>GSHMAGIFDLSGRKAIVTGGSKGIGAAIARALDKAGAT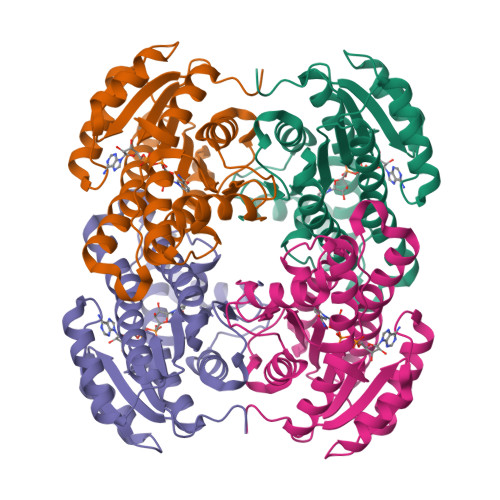VAIADLDVMAAQAVVAGLENGGFAVEVDVTKRASVDAAMQKAIDALGGFDLLCANAGVSTMRPAVDITDEEWDFNFDVNARGVFLANQIACRHFLASNTKGVIVNTASLAAKVGAPLLAHYSASKFAVFGWTQALAREMAPKNIRVNCVCPGFVKTAMQEREIIWEAELRGMTPEAVRAEYVSLTPLGRIEEPEDVADVVVFLASDAARFMTGQGINVTGGVRMD[4x]> MSERAYNFNAGPAALPLEVLERAQAEFVDYQHTGMSIMEMSHRGAVYEAVHNEAQARLLALLGNPTGYKVLFIQGGASTQFAMIPMNFLKEGQTANYVMTGSWASKALKEAKLIGDTHVAASSEASNYMTLPKLQEIQLQDNAAYLHLTSNETIEGAQFKAFPDTGSVPLIGDMSSDILSRPFDLNQFGLVYAGAQKNLGPSGVTVVIVREDLVAESPKHLPTMLRYDTYVKNNSLYNTPPSFGIYMVNEVLKWIEERGGLEGVQQANR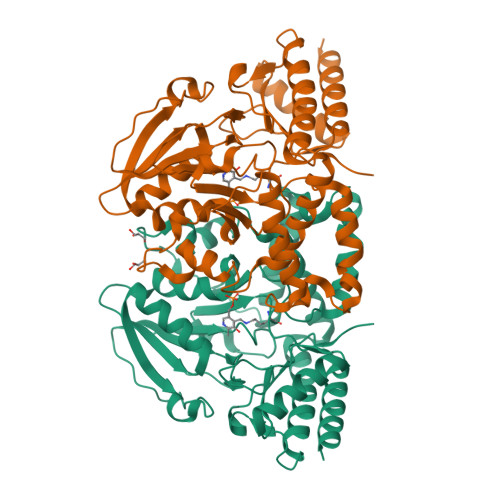KKASLIYDAIDQSGGFYRGCVDVDSRSDMNITFRLASEELEKEFVKASEQEGFVGLKGHRSVGGLRASIYNAVPYESCEALVQFMEHFKRSRG>[2x]AMKSYEIALIGNPNVGKSTIFNALTGENVYIGNWPGVTVEKKEGEFEYNGEKFKVVDLPGVYSL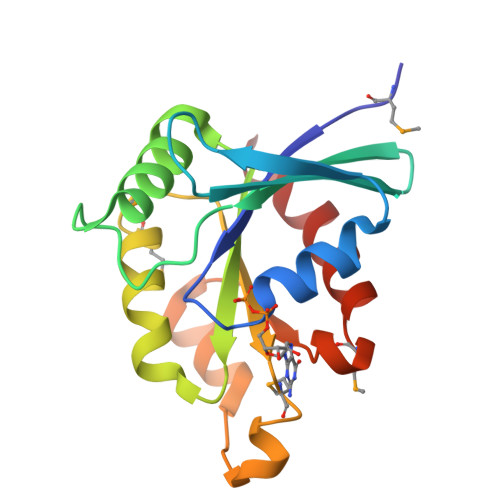TANSIDEIIARDYIINEKPDLVVNIVDATALERNLYLTLQLMEMGANLLLALNKMDLAKSLGIEIDVDKLEKILGVKVVPLSAAKKMGIEELKKAISIAVKDKK> ETGEATKSVSKTEHAEINIFSVASGHLYERMLN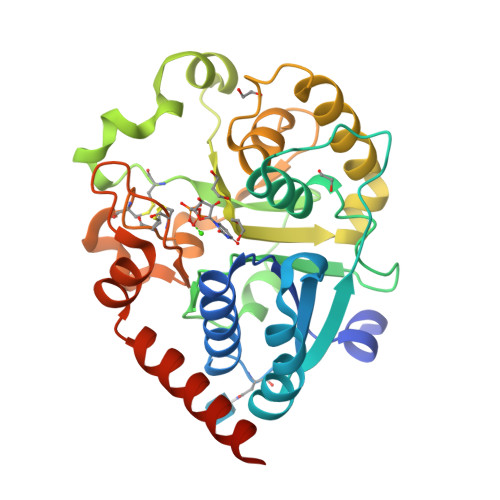IMMASVMHHTNHTVKFWFIEQFLSPSFKDFIPHMAAEYGFKYEMVTYKWPHWLRQQKEKQREIWGYKILFLDVLFPLSLDKVIFVDADQIVRTDMYDLVEHPLDGAPYGFAPMCDSRVEMEGYRFWKTGYWANYLKGKPYHISALYVVDLQRFRELAAGDRLRQQYHALSADPNSLANLDQDLPNHMQFTIPIATLPQEWLWCETWCSDETLKDARTIDLCNNPMTKEPKLDRARRQVPEWTKYDEEIAELARRVREGTKHHHHHH Human UDP-glucose dehydrogenase (hUGDH) catalyzes the oxidation of UDP-glucose into UDP-glucuronic acid, an essential substrate in the Phase II metabolism of drugs. hUGDH is a hexamer that exists in an equilibrium between an active (E) state and an inactive (EΩ) state, with the latter being stabilized by the binding of the allosteric inhibitor UDP-xylose (UDP-Xyl). hUGDH forms a hexamer arranged as a trimer of dimers, with each chain containing a NAD+ binding domain (NB domain) and a substrate binding domain (SB domain). The active site is located between the NB and SB domains within each chain, which are both flexible and undergo a rigid-body rotation to open the active site and bind substrate. What makes this allosteric is that the binding of UDP-Xyl changes the structure of the hexamer-building interface and increases the affinity between the adjacent subunits to form EΩ.12. This remarkable conformational change is controlled by a buried allosteric switch (the Thr131 loop/α6 helix) that responds to the identity of the C5 position of the nucleotide sugar bound in the active site.

To our surprise, the cryo-EM reconstruction showed that Escherichia coli, expressed hUGDH copurifies with a nucleotide sugar which stabilizes the hexamer in the EΩ conformation. Structural and biochemical analyses identify the nucleotide sugar as UDP-4-keto-xylose (UX4O), a structural analogue of UDP-Xyl that is produced in E. coli. Single particle cryo-EM data was collected and processed, revealing one major class corresponding to the EΩ conformation with a global resolution of 2.38 Å. This cryo-EM structure is similar to the previously published UDP-Xyl bound EΩ crystal structures. The lack of density for the NBexposed domains and weak density for the SBexposed domains in the cryo-EM structure of the EΩ state shows that they most likely exist as an ensemble of states in solution. The active sites of the cryo-EM hUGDH EΩ reconstruction reveal density for six nucleotide sugars that resemble the allosteric inhibitor UDP-Xyl. Similar to UDP-Xyl, these sugars stabilize the allosteric switch in the inhibited state which explains why we observe the EΩ hexamer. Two of the nucleotide sugars are located in the disordered NBexposed domains and have correspondingly weaker density. Modeling UX4O in the active site shows that the 4-keto-sugar fits the density and conserves most of the hydrogen bonding and packing interactions as previously observed for UDP-Xyl12. Based on the poor fit of UGDX to the density and the unfavorable steric clash, it is likely that the gem diol dehydrates in the active site and that UX4O is the bound form of the nucleotide.

>MFEIKKICCIGAGYVGGPTCSVIAHMCPEIRVTVVDVNESRINAWNSPTLPIYEPGLKEVVESCRGKNLFFSTNIDDAIKEADLVFISVNTPTKTYGMGKGRAADLKYIEACARRIVQNSNGYKIVTEKSTVPVRAAESIRRIFDANTKPNLNLQVLSNPEFLAEGTAIKDLKNPDRVLIGGDETPEGQRAVQALCAVYEHWVPREKILTTNTWSSELSKLAANAFLAQRISSINSISALCEATGADVEEVATAIGMDQRIGNKFLKASVGFGGSCFQKDVLNLVYLCEALNLPEVARYWQQVIDMNDYQRRRFASRIIDSLFNTVTDKKIAILGFAFKKDTGDTRESSSIYISKYLMDEGAHLHIYDPKVPREQIVVDLSHPGVSEDDQVSRLVTISKDPYEACDGAHAVVICTEWDMFKELDYERIHKKMLKPAFIFDGRRVLDGLHNELQTIGFQIETIGKKVSSKRIPYAPSGEIPKFSLQDPPNKKPKV[6x]>MTTLTRQDLNFGQVVADVLCEFLEVAVHLILYVREVYPVGIFQKRKKYNVPVQMSCHPELNQYIQDTLHCVKPLLEKNDVEKVVVVILDKEHRPVEKFVFEITQPPLLSISSDSLLSHV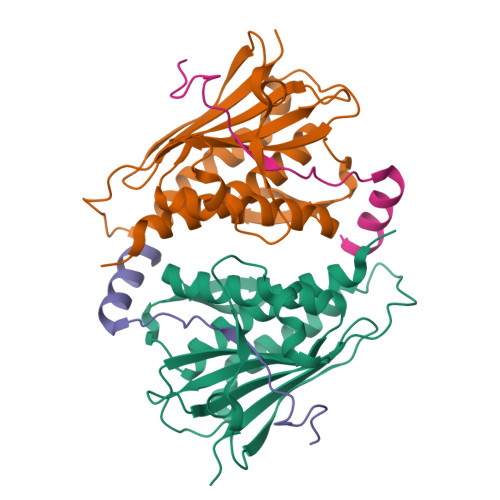EQLLAAFILKISVCDAVLDHNPPGCTFTVLVHTREAATRNMEKIQVIKDFPWILADEQDVHMHDPRLIPLKTMTSDILKMQLYVEERAHKGS[2x];>QDFPTRPLSRFIPWFPYDGSKLPLRPKRSPPVISEEAAEDVKQYLT[2x]>[2x]MAKIIWTRTDEAPLLATYSLKPVVEAFAATAGIEVETRDISLAGRILAQFPERLTEDQKVGNALAELGELAKTPEANIIKLPNISASVPQLKAAIKELQDQGYDIPELPDNATTDEEKDILARYNAVKGSAVNPVLREGNSDRRAPIAVKNFVKKFPHRMGEWSADSKTNVATMDANDFRHNEKSIILDAADEVQIKHIAADGTETILKDSLKLLEGEVLDGTVLSAKALDAFLLEQVARAKAEGILFSAHLKATMMKVSDPIIFGHVVRAYFADVFAQYGEQLLAAGLNGENGLAAILSGLESLDNGEEIKAAFEKGLEDGPDLAMVNSARGITNLHVPSDVIVDASMPAMIRTSGHMWNKDDQEQDTLAIIPDSSYA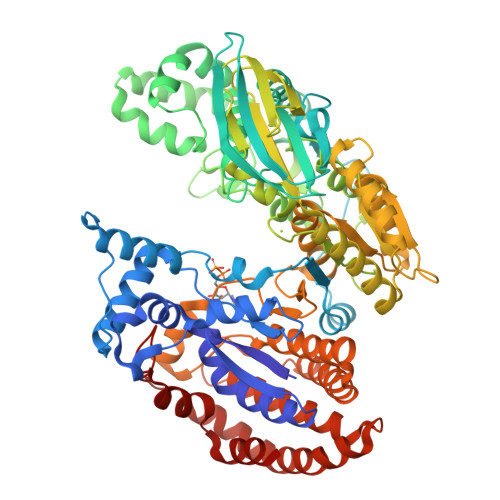GVYQTVIEDCRKNGAFDPTTMGTVPNVGLMAQKAEEYGSHDKTFRIEADGVVQVVSSNGDVLIEHDVEANDIWRACQVKDAPIQDWVKLAVTRSRLSGMPAVFWLDPERAHDRNLASLVEKYLADHDTEGLDIQILSPVEATQLSIDRIRRGEDTISVTGNVLRDYNTDLFPILELGTSAKMLSVVPLMAGGGLFETGAGGSAPKHVQQVQEENHLRWDSLGEFLALAESFRHELNNNGNTKAGVLADALDKATEKLLNEEKSPSRKVGEIDNRGSHFWLTKFWADELAAQTEDADLAATFAPVAEALNTGAADIDAALLAVQGGATDLGGYYSPNEEKLTNIMRPVAQFNEIVDALKK Cytohesins comprise a metazoan Arf GEF family with four mammalian paralogs (Grp1, ARNO, and cytohesins-1/4) that function in receptor signaling, endocytic trafficking, and cell adhesion/migration (Chardin et al., 1996, Fuss et al., 2006, Hafner et al., 2006, Hickman et al., 2018, Ito et al., 2018, Kolanus et al., 1996, Li et al., 2012, Mohanan et al., 2018, Ogasawara et al., 2000, Rafiq et al., 2017). All cytohesins share a common architecture comprised of a heptad repeat coiled coil (CC) domain, the Sec7 domain, and a pleckstrin-homology (PH) domain. The PH domain binds phosphatidyl inositol 3,4,5-trisphosphate (PIP3) and/or phosphatidyl inositol 4,5-bisphosphate (PIP2) (Chardin et al., 1996, Kavran et al., 1998, Klarlund et al., 1997), with affinities, specificities and spatiotemporal distributions dependent on splice variation in the phosphoinositide-binding pocket (Cronin et al., 2004, Klarlund et al., 2000, Ratcliffe et al., 2018). Two autoinhibitory elements, the Sec7-PH linker and C-terminal helix/polybasic region (CtH/PBR), strongly suppress GEF activity by occluding the active site in the Sec7 domain (DiNitto et al., 2007).

To address these issues and gain additional insight, the structural organization and extent of conformational variability of Grp114-399 dimers was independently investigated by single-particle NS-EM. Unsupervised reference-free classification of ∼10,000 manually picked particles from 500 micrographs yielded 53 good quality classes representing ∼6,500 particles. Attempts to generate a 3D reconstruction with visually selected particle classes were unsuccessful, suggesting potential conformational heterogeneity. To explore this possibility, the 2D class averages were systematically compared with 3D volume projections over the range of possible views for each model in the MultiFoXS pools. The 2D analysis suggested that conformational similarity of best scoring models might improve selection of classes for 3D reconstruction. For two class sets corresponding to compact or intermediate best scoring models, 3D volumes could be built and refined. Automated docking of the MultiFoXS pools with the refined 3D volumes selected best scoring models having relatively compact conformations similar to the more compact models in the six-state MultiFoXS ensembles. The low resolution of ∼53 Å for the refined 3D volumes likely reflects conformational heterogeneity in addition to negative staining. Flexibility in the CC-Sec7 linker is the main source of conformational variability, with a secondary contribution from hinge conformers that does not appear to be strongly influenced by dimerization. Although the analyses are most consistent with an antiparallel CC topology, the resolution is not sufficient to definitively exclude parallel or mixed topologies.

>MGHHHHHHGSPEDLSLEEREELLDIRRRKKELIDDIERLKYEIAEVMTEIDNLTSVEESKYTQRNAQIAMGRKKFNMDPKKGIQFLIENDLLQSSPEDVAQFLYKGEGLNKTVIGDYLGERDDFNIKVLQAFVELHEFADLNLVQALRQFLWSFRLPGEAQKIDRMMEAFASRYCLCNPGVFQSTDTCYVLSFAIIMLNTSLHNHNVRDKPTAERFITMNRGINEGGDLPEELLRNLYESIKNEPFKIPEDDGNDLTYTFFNPDREGWLLKLGGRVKTWKRRWFILTDNCLYYFEYTTDKEPRGIIPLENLSIREVEDPRKPNCFELYNPSHKGQVIKACKTEADGRVVEGNHVVYRISAPSPEEKEEWMKSIKASISRDPFYDMLATRKRRIANKK[2x]> GSMTEADVNPKAYPLADAHLTKKLLDLVQQSCNYKQLRKGANEATKTLNRGISEFIVMAADAEPLEIILHLPLLCED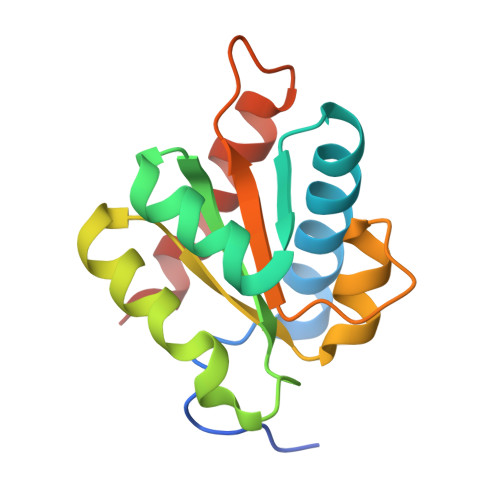KNVPYVFVRSKQALGRACGVSRPVIACSVTIKEGSQLKQQIQSIQQSIERLLV The human (h) TR exists in two isoforms, hTRα (NR1A1), and hTRβ (NR1A2). hTRα is expressed at higher levels in heart and plays a major role in regulation of heart rate, whereas TRβ is the predominant isoform that is expressed in the liver and pituitary and is involved with hepatic cholesterol metabolism and regulation of metabolic rate. Thyroid receptor (TR) activation occurs when an agonist ligand such as TH or similar compounds binds to a hydrophobic pocket in the core of its ligand-binding domain (LBD). This causes conformational changes which allow DNA bound receptors to interact with coactivators, mediating transcription.

In the second crystal form (C2 space group) Arg 228 is in another non-productive conformation (in white) which is an intermediate between two conformations of the same residue found in the first crystal form. Differential positioning of the Arg228 side chain is related to hydrogen bond with the Ser277 carbonyl group that flips the Arg228 side chain into an alternative conformation. To compensate this conformational change, a water molecule (W343) bridges the Arg228 side chain and the GC-1 carboxylate group. This weakens direct interaction with Arg228 and forces GC-1 into a new conformation which involves re-orientation of its carboxyl group. First, the GC-1 oxyacetic acid ester oxygen forms a hydrogen bond with the main chain amino group of TRα specific Ser277 residue. The Ser277 side chain hydroxyl participates in a hydrogen bond interaction with the Ile221 main chain carbonyl group, which is not available to Asn331 in hTRβ. This means that Ser277 fails to engage in a hydrogen bond contact with Arg228 analogous to that observed between Asn331 and Arg282. Thus, Arg228 is not anchored by contacts with the subtype specific residue. In the non-productive conformations GC-1 maintains the interaction with Ser277 but the strong interaction of GC-1 with Arg228 is lost, giving way to a hydrogen bond of this residue with the main carbonyl of Ser277. While hTRβ Arg282 binds to the ligand in a single conformation, hTRα Arg228 has the potential to flip away from the ligand in non-productive conformations, resulting in loss of an important interaction for the stabilization the ligand.

> ARGSHMEEMIRSLQQRPEPTPEEWDLIHIATEAHRSTNAQGSHWKQRRKFLPDDIGQSPIVSMPDGDKVDLEAFSEFTKIITPAITRVVDFAKKLPMFSELPCEDQIILLKGCCMEIMSLRAAVRYDPESDTLTLSGEMAVKREQLKNGGLGVVSDAIFELGKSLSAFNLDDTEVALLQAVLLMSTDRSGLLCVDKIEKSQEAYLLAFEHYVNHRKHNIPHFWPKLLMKVTDLRMIGACHASRFLHMKVECPTELFPPLFLEVFEDQEV> HPQG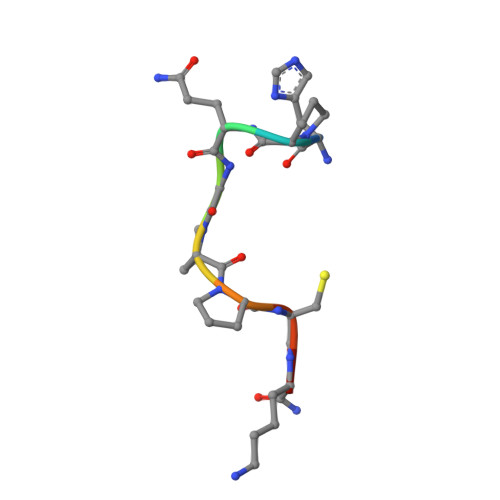PPCKX(3R)-4-{[4-(4-cyano-3-methylphenoxy)phenyl]acetyl}morpholine-3-carboxylic acid | C21 H20 N2 O5 | 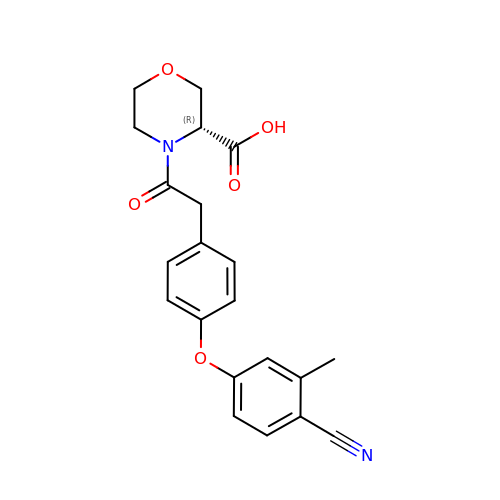AJUGJYIFDAVOIF-LJQANCHMSA-N>MGSSHHHHHHSQDPNSMLSVGATTTATRLTGWGRTAPSVANVLRTPDAEMIVKAVARVAESGGGRGAIARGLGRSYGDNAQNGGGLVIDMTPLNTIHSIDADTKLVDIDAGVNLDQLMKAALPFGLWVPVLPGTRQVTVGGAIACDIHGKNHHSAGSFGNHVRSMDLLTADGEIRHLTPTGEDAELFWATVGGNGLTGIIMRATIEMTPTSTAYFIADGDVTASLDETIALHSDGSEARYTYSSAWFDAISAPPKLGRAAVSRGRLATVEQLPAKLRSEPLKFDAPQLLTLPDVFPNGLANKYTFGPIGELWYRKSGTYRGKVQNLTQFCHPLDMFGEWNRAYGPAGFLQYQFVIPTEAVDEFKKIIGVIQASGHYSFLNVFKLFGPRNQAPLSFPIPGWNICVDF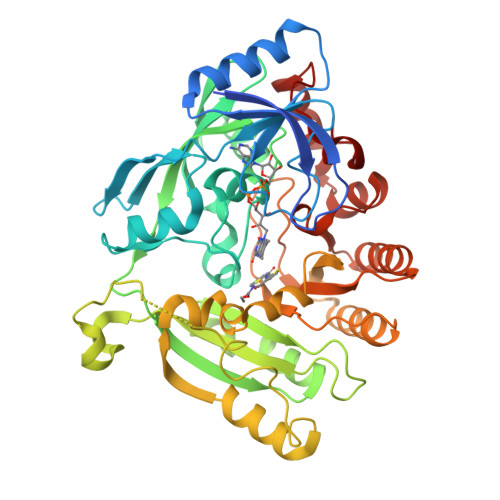PIKDGLGKFVSELDRRVLEFGGRLYTAKDSRTTAETFHAMYPRVDEWISVRRKVDPLRVFASDMARRLELL[2x]>MLDNPFIGAIGYVNPDWATNVISQANQTADPTLAAQMRKVATYSTAVWLDRIAAITAGRGLRGHLDEALRQMQQAGQPVVITLVIYDLPNRDCSAAASNGELLVAQNGLARYKAEFIDPIVAILSDPRYAGLRIVTIIEPDSLPNLVTNLSIPACAEAQNAYIEGIRYAVNRLRTIPNVYIYLDIAHSGWLGWDNNFNGAVNLYTQVVQGMDQGFNSIDGFITNVANYTPLEEPYLPDPNLTIAGQPVRSASFYEWNPYFDELDYALALRNAFIGRGFPSTIGMLIDTSRNGWGGCSYGRCRPTGPSSDTSSVNAYVDGSRVDRRYHRGNWCNQAGGIGERPQAAPRSGIDA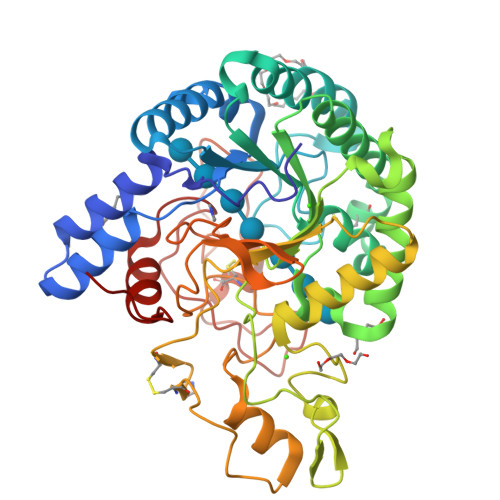YVWVKPPGESDGVSQPGIVDPDDPNKKFDPMCDPNGQSRYNSAYPTGALPNAPHAGRWFPQQFEILVRNAYPPIQP[3x]The enzyme, therefore, turned out to be scyllo-inositol dehydrogenase with L-glucose dehydrogenase activity (P. laeviglucosivorans scyllo-inositol dehydrogenase; Pl-scyllo-IDH). Further analysis showed that the enzyme oxidized L-glucose to L-glucono-1,5-lactone as the first step in the pathway for L-glucose metabolism. Pl-scyllo-IDH formed a homo-tetrameric structure in the asymmetric unit, and this structure was considered the biologically relevant form, since a similar unit has been observed for myo-IDH from B. subtilis and GFOR from Zymmomonas mobilis. The N-terminal domain adopted a Rossmann fold motif for the binding of NAD+, and the C-terminal domain bound substrate.

Since Pl-scyllo-IDH also oxidizes scyllo-inositol and myo-inositol, the complex structures of Pl-scyllo-IDH with scyllo-inosose and myo-inositol were also determined. Both inositols bound to the catalytic site in essentially the same manner as each other, where residues K106, Y135, Y163, E165, R178, D191, and H318 formed hydrogen bonds with the hydroxyl oxygen of the sugar. All six inositol hydroxyl oxygens were involved in hydrogen bonds, including bipartite and tripartite bonds making for a total of eleven bonds. On the other hand, in the case of the inositols, R178 was positioned inside the active site in order to be able to interact with the substrates. In the case of myo-inositol binding, based on the shape of the electron density map, the 4’-OH formed a hydrogen bond with K106, which suggests that the reaction product is L-epi-2-inosose. myo-IDH from B. subtilis is known to oxidize 2ʹ-OH of myo-inositol resulting in scyllo-inosose production. Therefore, Pl-scyllo-IDH may have a different regioselectivity with myo-IDH toward myo-inositol. Therefore, L-epi-2-inosose can be a substrate for Pl-scyllo-IDH, and the enzyme is highly possible to be the first enzyme catalyzing reversible oxidation of myo-inositol to L-epi-2-inosose. Based on the crystal structure of Pl-scyllo-IDH complexed with inositols, side chains of D191 and H195 were found to be oriented to K106; on the other hand, in the structure complexed with L-glucono-1,5-lactone, the side chain of D191 was parallel to the sugar plane and extended outward from the active site. The corresponding distances in the myo-inositol and scyllo-inosose complexes were 2.8 Å and 3.1 Å, respectively, and the relative positions of NAD+ and the inositols were the same as those seen in the lactone complex.

>[4x]MSNAEKALGVALIGTGFMGKCHAMAWRNVATAFGGLPPRLEVLADMPADKAHSLASSFGFARGTADWREAVSDPAVDVVSITTPNGLHREMAEAALAAGKHVWLEKPMALSVEDAQAMEAAARASDRRTIIGYNYTRSPAFRAAVDLIAEGAIGRPIHFRGMYDEDYMADPDLPWSWRLTRKDGGLGALGDLGCHLVSVMVSLMGPVARVYAQADTVITDRPHQGGTARVENEDQAQALIRFASGTSGEFSCSRVARGYRCRLAWEVQGTEGTLRFDQERMNELWLYQPGRPEIDGFRRILTGPAQPGFAAFCPGGGHNFGFNEQKVVEAEMLRQAIAGRGKAWPDFTDGLTIERVIHGMATSAQTGQPVNFLEHHHHHH> MFIENKPGEIELLSFFESEPVSFERDNISFLYTAKN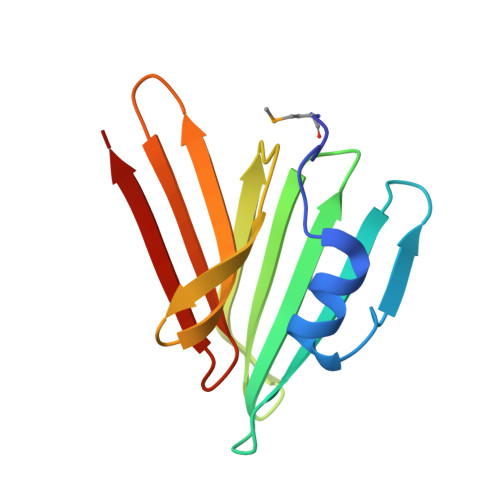KCGLSVDFSFSVVEGWIQYTVRLHENEILHNSIDGVSSFSIRNDNLGDYIYAEIITKELINKIEIRIRPDIKIKSSSVIR>GPMFEARLVQGSILKKVLEALKDLINEACWDISSSGVNLQSMDSSHVSLVQLTLRSEGFDTYRCDRNLAMGVNLTSMSKILKCAGNEDIITLRAEDNADTLALVFEAPNQEKVSDYEMKLMDLDVEQLGIPEQEYSCVVKMPSGEFARICRDLSHIGDAVVISCAKDGVKFSASGELGNGNIKLSQTSNVDKEEEAVTIEMNEPVQLTFALRYLNFFTKATPLSSTVTLSMSADVPLVVEYKIADMGHLKYYLAPKIEDEEGS[3x];>[3x]SSMRKICTYFHRKS

The CRL4Cdt2 ubiquitin ligase complex is an essential regulator of cell-cycle progression and genome stability, ubiquitinating substrates such as p21, Set8, and Cdt1, via a display of substrate degrons on proliferating cell nuclear antigens (PCNAs). In contrast, CRL4Cdt2 recognizes Cdt1 when bound to the proliferating cell nuclear antigen (PCNA) trimer, through a binding motif (PIP box) in its N-terminal end. Unexpectedly, we found a PIP box in the C-terminal end of Cdt2, and showed that it directly mediates interaction of Cdt2 with PCNA. X-ray crystallographic structures of PCNA bound to Cdt2PIP and Cdt1PIP show that the peptides occupy all three binding sites of the trimeric PCNA ring.

Our search revealed a PIP box sequence from amino acids 706 to 713 in the C-terminus of Cdt2. To confirm that this PIP box motif in Cdt2 interacts directly with PCNA, and to quantify that interaction, we synthesized the peptide corresponding to the human Cdt2 PIP box (704-717) (SSMRKICTYFHRKS) with a carboxytetramethylrhodamine fluorescent label at the N-terminus (Cdt2PIP) and characterized its binding to recombinant PCNA, by fluorescence polarization (FP). Cdt2PIP binds PCNA with high affinity (57 ± 3 nM). The corresponding Cdt2PIP-3A peptide showed practically no detectable binding to PCNA in the same assay, suggesting that the Cdt2 PIP box binds PCNA in a manner very similar to other known PCNA complexes with PIP box peptides. To confirm the binding mode of the Cdt2PIP and Cdt1PIP peptides to PCNA, we determined the crystal structure of both complexes by X-ray crystallography, to a 3.5- and 3.4-Å resolution, respectively. PCNA adopts its well-characterized trimer conformation, with one peptide bound per monomer. Some notable differences in the binding mode are the conserved Phe713/Phe11 side-chain ring that rotates 180 degrees between the two structures and the Tyr712/Phe10 that repositions so as to extend more towards a hydrophilic environment in Cdt2. The Ile709 and Val7 side chains occupy a similar space in the hydrophobic recognition pocket. The average buried area upon the binding of the Cdt2 peptide is 692 ± 6 Å2 and average calculated energy of binding is −13 ± 0.2 kcal·mol−1, whereas the average buried area upon the binding of the Cdt1 peptide is 650 ± 4 Å2 and average calculated energy of binding is −8.3 ± 0.5 kcal·mol−1; these confirm the tighter binding of the Cdt2 peptide to PCNA. The affinity of the Cdt2PIP peptide for PCNA is similar to that reported for the tightly binding p21 PIP box peptide (50–85 nM), as it was confirmed in our assays (RRQTSMTDFYHSKR, 36 ± 2 nM).In acrylate metabolism and detoxification, AcuH is functional in both the AcuN-AcuK pathway and the PrpE-AcuI pathway. It can catalyze acryloyl-CoA hydration in the AcuN-AcuK pathway and the branching of the PrpE-AcuI pathway. Conserved domain analysis suggests that RdAcuH belongs to the crotonase superfamily (1.07e-74) and is predicted as an enoyl-CoA hydratase (6.64e-150). The activity assay results showed that RdAcuH has acryloyl-CoA hydratase activity and can catalyze acryloyl-CoA to 3-HP-CoA.

With the enoyl-CoA hydratase from R. norvegicus as a model, the structure of RdAcuH was solved at the resolution of 1.9 Å. The overall structure of RdAcuH is a dimer of trimers in an asymmetric unit of the crystal, in which three monomers associate end to end to form a tight trimer, and two trimers associate back to back to form a dimmer. There are few strong interactions between these two trimers. Thus, the dimer should result from crystal packing. Each RdAcuH subunit contains two domains, an N-terminal domain (NTD) and a C-terminal domain (CTD). The NTD adopts a typical spiral crotonase fold which is organized by two perpendicular β-sheets. There are three active centers in each trimer and each active center is located between the NTD of a subunit and the CTD of the neighboring subunit. Because RdAcuH and the enoyl-CoA hydratase from R. norvegicus have high similarity in their sequences and structures, we found that the corresponding residues of these two glutamates in RdAcuH are Glu112 and Glu132 according to the sequence and structure alignment. Biochemical analysis showed that mutations on each of the glutamates to alanine resulted in the inactivation of RdAcuH. Like the enoyl-CoA hydratase from R. norvegicus, there should be a water molecule in the position of the acetic acid molecule that acts as a catalytic water, and the carboxylates of Glu112 and Glu132 are expected to be ionized under a neutral condition.

>[6x]MAYETIIVEVEDHVALITLNRPDALNALNDQLLSELVKALEDAQNNDKVRCIVITGSEKAFAAGADIKMMSEKSFVDVFAGDLFGPEAEGIMRIRKPIIAAVSGYALGGGCELAMMCDFIICSDTAKFGQPEINLGVIAGMGGSQRLTRFIGKSKSMDMNLTGRFMDAEEAERSGLVSRVVPAKKLMEETMTAAQKIAEKSMIAVMAVKEAVNRSYEVPLREGLLFERRVFQSLFATEDQKEGMSAFAEKREAQFRDK>[4x]GSHMGVGSVAALLTVVFYIAAVMATNLYGATFPEWFGDLSKSLYTLFQVMTLDSWSMGIVRPVMNVHPNAWVFFIPFIMLTTFTVLNLFIGIIVDAMAITKEQEEEAKTGHHQEPISQTLLHLGDRLDRIEKQLAQNNELLQRQQPQKK

Prokaryotic sodium channels are homotetramers, in which each monomer contains six transmembrane segments and is homologous to a single eukaryotic pseudorepeat. As with the eukaryotic channels, their S1–S4 segments form the voltage sensors, and the S5–S6 segments from each polypeptide chain associate to form an eight‐helix bundle that constitutes the pore. The selectivity filter (SF), which determines the channel's Na+ permeability over other cations, is formed by the close association of the P loops from each of the polypeptide chains.

To specifically test the role of the E178 residue located at the extracellular end of the SF in the selectivity and translocation properties of NavMs, we mutated its SF from LESWSM to LDSWSM. This mutation changes the residue near the NaI site from a glutamic acid to the shorter aspartic acid, but does not alter the net charge of the SF. The crystal structure of the E178D mutant showed considerable differences from the wild‐type channel local to the site of the mutation: the methylene group of the glutamic acid was missing, producing a side chain that projected to a lesser extent into the SF, as expected, and the site at NaI was completely devoid of ordered electron density, suggesting that it was unoccupied by an ion. The alteration in the protein structure caused by removal of the methylene group of E178 exposes a positive region of the polypeptide backbone adjacent to the site where the top sodium ion is located in the wild‐type protein; this likely contributes to why an equivalent sodium ion is not seen adjacent to this position in the mutant. Soaking the crystals in calcium, which might have been expected to produce additional density if the SF had become calcium‐selective, produced a similar result: no density was seen in the region of the D178 residue (data not shown). Relative to wild‐type, the mutant has a more electropositive region (denoted by the circle in Fig 3B right) at the top of the SF, due to the exposure of the backbone nitrogen of residue S179 when the longer side chain of residue E178 is replaced with the shorter side chain in the mutant; this could tend to inhibit cations from binding at this site, consistent with measured decreased current densities. Sodium ions are shown as cyan spheres; only 2 are present in the mutant, instead of the 3 seen in the wild‐type, with the top sodium missing in the mutant. The current density of the E178D mutant channel was 15‐times less than that found in the wild‐type channel measured under sodium‐only conditions (11.4 ± 3 vs. 165 ± 21 pA/pF). As the structure demonstrates that there is one less binding site in the mutant channel than in the wild‐type structure, this could be consistent with fewer ions passing through the channel per unit of time, and therefore a lower current density. K+, Ca2+ and Ba2+ conductances were detected (albeit at lower levels) in addition to Na+ and Li+.> GPAMQSVSNDEVKDQLADNGGNSAYDNNDDAVEVGKSMENVAMPVVDSENVSVVKKFYETDAAKEEKEAALVTYNNTYSLSKGIDLAEKDGKDFDVSASLSGTVVKAEKDPVLGYVV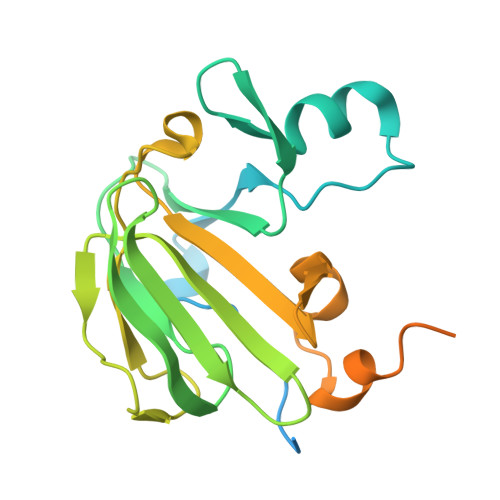EVEHADGLSTVYQSLSEVSVEQGDKVKQNQVIGKSGKNLYSEDSGNHVHFEIRKDGVAMNPLNFMDKPVSSIEKAATQETEESIQQSSEKKDGSTEKGTEEKSGEKKDDSTDKSGSKESSTTEDTEQS>MASGSCQGCEEDEETLKKLIVRLNNVQEGKQIETLVQILEDLLVFTYSEHASKLFQGKNIHVPLLIVLDSYMRVASVQQVGWSLLCKLIEVCPGTMQSLMGPQDVGNDWEVLGVHQLILKMLTVHNASVNLSVIGLKTLDLLLTSGKITLLILDEESDIFMLIFDAMHSFPANDEVQKLGCKALHVLFERVSEEQLTEFVENKDYMILLSALTNFKDEEEIVLHVLHCLHSLAIPCNNVEVLMSGNVRCYNIVVEAMKAFPMSERIQEVSCCLLHRLTLGNFFNILVLNEVHEFVVKAVQQYPENAALQISALSCLALLTETIFLNQDLEEKNENQENDDEGEEDKLFWLEACYKALTWHRKNKHVQEAACWALNNLLMYQNSLHEKIGDEDGHFPAHREVMLSMLMHSSSKEVFQASANALSTLLEQNVNFRKILLSKGIHLNVLELMQKHIHSPEVAESGCKMLNHLFEGSNTSLDIMAAVVPKILTVMKRHETSLPVQLEALRAILHFIVPGMPEESREDTEFHHKLNMVKKQCFKNDIHKLVLAALNRFIGNPGIQKCGLKVISSIVHFPDALEMLSLEGAMDSVLHTLQMYPDDQEIQCLGLSLIGYLITKKNVFIGTGHLLAKILVSSLYRFKDVAEIQTKGFQTILAILKLSASFSKLLVHHSFDLVIFHQMSSNIMEQKDQQFLNLCCKCFAKVAMDDYLKNVMLERACDQNNSIMVECLLLLGADANQAKEGSSLICQVCEKESSPKLVELLLNSGSREQDVRKALTISIGKGDSQIISLLLRRLALDVANNSICLGGFCIGKVEPSWLGPLFPDKTSNLRKQTNIASTLARMVIRYQMKSAVEEGTASGSDGNFSEDVLSKFDEWTFIPDSSMDSVFAQSDDLDSEGSEGSFLVKKKSNSISVGEFYRDAVLQRCSPNLQRHSNSLGPIFDHEDLLKRKRKILSSDDSLRSSKLQSHMRHSDSISSLASEREYITSLDLSANELRDIDALSQKCCISVHLEHLEKLELHQNALTSFPQQLCETLKSLTHLDLHSNKFTSFPSYLLKMSCIANLDVSRNDIGPSVVLDPTVKCPTLKQFNLSYNQLSFVPENLTDVVEKLEQLILEGNKISGICSPLRLKELKILNLSKNHISSLSENFLEACPKVESFSARMNFLAAMPFLPPSMTILKLSQNKFSCIPEAILNLPHLRSLDMSSNDIQYLPGPAHWKSLNLRELLFSHNQISILDLSEKAYLWSRVEKLHLSHNKLKEIPPEIGCLENLTSLDVSYNLELRSFPNEMGKLSKIWDLPLDELHLNFDFKHIGCKAKDIIRFLQQRLKKAVPYNRMKLMIVGNTGSGKTTLLQQLMKTKKSDLGMQSATVGIDVKDWPIQIRDKRKRDLVLNVWDFAGREEFYSTHPHFMTQRALYLAVYDLSKGQAEVDAMKPWLFNIKARASSSPVILVGTHLDVSDEKQRKACMSKITKELLNKRGFPAIRDYHFVNATEESDALAKLRKTIINESLNFKIRDQLVVGQLIPDCYVELEKIILSERKNVPIEFPVIDRKRLLQLVRENQLQLDENELPHAVHFLNESGVLLHFQDPALQLSDLYFVEPKWLCKIMAQILTVKVEGCPKHPKGIISRRDVEKFLSKKRKFPKNYMTQYFKLLEKFQIALPIGEEYLLVPSSLSDHRPVIELPHCENSEIIIRLYEMPYFPMGFWSRLINRLLEISPYMLSGRERALRPNRMYWRQGIYLNWSPEAYCLVGSEVLDNHPESFLKITVPSCRKGCILLGQVVDHIDSLMEEWFPGLLEIDICGEGETLLKKWALYSFNDGEEHQKILLDDLMKKAEEGDLLVNPDQPRLTIPISQIAPDLILADLPRNIMLNNDELEFEQAPEFLLGDGSFGSVYRAAYEGEEVAVKIFNKHTSLRLLRQELVVLCHLHHPSLISLLAAGIRPRMLVMELASKGSLDRLLQQDKASLTRTLQHRIALHVADGLRYLHSAMIIYRDLKPHNVLLFTLYPNAAIIAKIADYGIAQYCCRMGIKTSEGTPGFRAPEVARGNVIYNQQADVYSFGLLLYDILTTGGRIVEGLKFPNEFDELEIQGKLPDPVKEYGCAPWPMVEKLIKQCLKENPQERPTSAQVFDILNSAELVCLTRRILLPKNVIVECMVATHHNSRNASIWLGCGHTDRGQLSFLDLNTEGYTSEEVADSRILCLALVHLPVEKESWIVSGTQSGTLLVINTEDGKKRHTLEKMTDSVTCLYCNSFSKQSKQKNFLLVGTADGKLAIFEDKTVKLKGAAPLKILNIGNVSTPLMCLSESTNSTERNVMWGGCGTKIFSFSNDFTIQKLIETRTSQLFSYAAFSDSNIITVVVDTALYIAKQNSPVVEVWDKKTEKLCGLIDCVHFLREVTVKENKESKHKMSYSGRVKTLCLQKNTALWIGTGGGHILLLDLSTRRLIRVIYNFCNSVRVMMTAQLGSLKNVMLVLGYNRKNTEGTQKQKEIQSCLTVWDINLPHEVQNLEKHIEVRKELAEKMRRTSVE[2x]

Leucine-rich repeat kinase 2 (LRRK2) is a highly pursued drug target for Parkinson’s disease (PD), which is the second most common neurodegenerative disease projected to affect 17.5 million people by 20401. LRRK2 is a 286-kDa protein containing seven domains (ARM, ANK, LRR, ROC, COR, KIN, and WD40) with kinase and GTPase activities. Autosomal dominant LRRK2 mutations with higher kinase activity are leading genetic causes of both familial and sporadic late-onset PD cases. Here we report high-resolution cryo-EM structures of LRRK2 in complex with a panel of small molecules, including two type I (LRRK2-IN-1 and GNE-7915) and three type II inhibitors (rebastinib, ponatinib, and GZD-824).

Following a similar purification approach, type II inhibitors were mixed with full-length LRRK2 protein in an ATP-free buffer before cryo-EM analysis. Both LRRK2 monomer and dimer exist in the same grid, and we were able to resolve LRRK2–ponatinib, LRRK2–GZD-824, LRRK2–rebastinib complexes at nominal overall resolutions of 3.4, 3.6, and 3.7 Å, respectively. GZD-824 and ponatinib are analogous compounds and bind to LRRK2 in a similar manner. Specifically, the main chains of A1950 and D2017 and the side chain of E1920 form polar interactions with nitrogen and oxygen atoms in all three small molecules. Our structures show that Ala2016 directly interacts with all three type II inhibitors tested here, with its side chain pointing towards the inhibitors, but not ATP. The binding of type II inhibitors resulted in the structural re-arrangement of the ATP-binding site. Furthermore, rebastinib, ponatinib, and GZD-824 occupy the position that was otherwise taken by the alpha helix of the activation segment. Tyr2018 in the “DYG” motif rotates and interacts with type II inhibitors, and Lys1906 and Glu1920 form a salt bridge. Additionally, the αC helix moves towards the ATP-binding site and interacts with the small molecules. The LRRK2–GZD824, LRRK2–rebastinib, and LRRK2–ponatinib complexes provide structural templates for designing LRRK2-specific type II inhibitors.> GAGCAGACAAG;> ACTCCACTCA;> CTAGT;> TCTGAGTGGTGTCTGC

In this work, we exhaustively probe the ability of all 36 immobile HJ sequences to form DNA crystals in two different designed systems. Three separate self-assembling DNA crystal systems are described in this report: the “4 × 5” and “4 × 6” designs (collectively referred to as the 4 × N systems), and a third construct with a “scrambled” sequence variant of the 4 × 6 lattices. Self-assembly was mediated by three constituent oligonucleotides: (S1) containing four sequence repeats of either 5 or 6 bases; (S2) composed of 21 bases containing complementary regions to both (S1); and (S3) which forms the second junction crossover. The HJ serves as the fundamental component at the core of each unit, and the ultimate assembly of the full lattice is facilitated by the complementary 2-base sticky ends that tail each duplex.

The 4 × 5 system robustly crystallized with 75% of the junctions, and we obtained crystals in all but 9 of 36 sequences. In the 4 × 5 system, J25 and J34, both displaying P32 symmetry, crystallized in 50 mM Tris pH = 8.0 buffer containing cobalt hexamine (CoH18N6) and 10 mM MgCl2, and 50 mM HEPES pH = 7.5 with 20 mM MgCl2, respectively. Only cobalt could account for the different peaks in the Fo–Fc maps in J25, whereas in J34, and J22 and J23 in the 4 × 6 and 4 × 6 scramble systems, respectively, contained Mg2+. The modeled ions were readily superimposable, and well-coordinated at Pos1 & 2. Of the resulting structures, 18 exhibited P32 symmetry with average cell dimensions a = b = 68.85 Å c = 60.09 Å, with only nine retaining the original P3221 symmetry with average cell edges a = b = 68.17 Å c = 60.60 Å. Although the cell parameters between the two symmetries were virtually indistinguishable, the differences between the periodicity of the lattices is dramatic, with vastly different cavity sizes.>[2x]AKIGLFFGSNTGKTRKVAKSIKKRFDDETMSDALNVNRVSAEDFAQYQFLILGTPTLGEGELPGLSS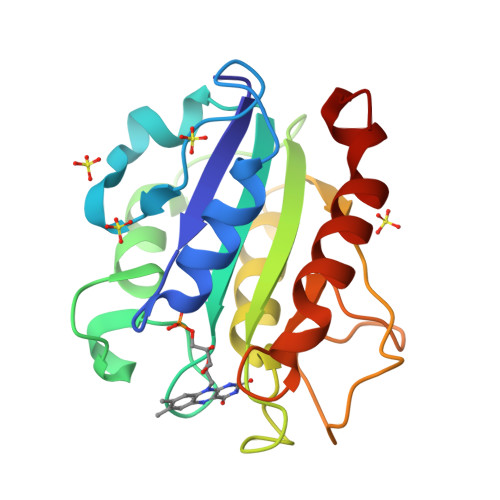DAENESWEEFLPKIEGLDFSGKTVALFGLGDQVGYPENYLDALGELYSFFKDRGAKIVGSWSTDGYEFESSEAVVDGKFVGLALDLDNQSGKTDERVAAWLAQIAPEFGLSL>MDEKKLFLKALKKKFEGEDPDEKYTNFYCFGGWEQSARKKEFTEYAKKAAEKRGGIPFYNPDIGVPLGQRKLMAYRVSGTDAYVEGDDLHFVNNAAIQQMVDDIKRTVIVGMDTAHAVLEKRLGVEVTPETINEYMEAINHALPGGAVVQEHMVEVHPGLVEDCYAKIFTGDDNLADELDKRILIDINKEFPEEQAEQLKSYIGNRTYQVNRVPTIVVRTCDGGTVSRWSAMQIGMSFISAYKLCAGEAAIADFSYAAKHADVIEMGTIMPARRARGPNEPGGVAFGTFADIVQTSRVSDDPANVSLEVIAGAAALYDQVWLGSYMSGGVGFTQYATAAYTDDILDDFVYYGMEYVDDKYGICGTKPTMDVVRDISTEVTLYSLEQYEEYPTLLEDHFGGSQRAAVAAAAAGCSTAFATGNSNAGINGWYLSQILHKEAHSRLGFYGYDLQDQCGASNSLSIRSDEGLIHELRGPNYPNYAMNVGHQPEYAGIAQAPHAARGDAFCTNPLIKVAFADKDLAFDFTSPRKSIAAGALREFMPEGERDLIIPAGK[4x];>[4x]MPMYEDRIDLYGADGKLLEEDVPLEAISPLKNPTIANLVSDVKRSVAVNLAGIEGSLRKAALGGKSNFIPGREVELPIVENAEAIAEKVKKLVQTSEDDDTNIRLINNGQQILVQVPTTRMGVAADYTVSALVTGAAVVQAIIDEFDVDMFDANAVKTAVMGRYPQTVDFTGANLSTLLGPPVLLEGLGYGLRNIMANHVVAITRKNTLNASALSSILEQTAMFETGDAVGAFERMHLLGLAYQGLNANNLLFDLVKENGKGTVGTVIASLVERAVEDGVVKVAREMNSGYKVYEPADWALWNAYAATGLLAATIVNVGAARAAQGVASTVLYYNDILEYETGLPGVDFGRAMGTAVGFSFFSHSIYGGGGPGIFHGNHVVTRHSKGFALPCVAAAMCLDAGTQMFSVEKTSGLIGSVYSEIDYFREPIVNVAKGAAEVKDQL;>MSYKAQYTPGETQIAENRRKHMDPDYEFRKLREVSDEDLVKVLGHRNPGESYKSVHPPLDEMDFEEDIVRDMVEPIQGAKEGVRVRYIQFADSMYNAPAQPYDRARTYMWRYRGVDTGTLSGRQVIEMRELDLEGVSKELVETELFDPATTGIRGATVHGHSLRLDENGLMFDALQRYVFDEEKGHVVYVKDQVGRPLDEPVDMGQPLGE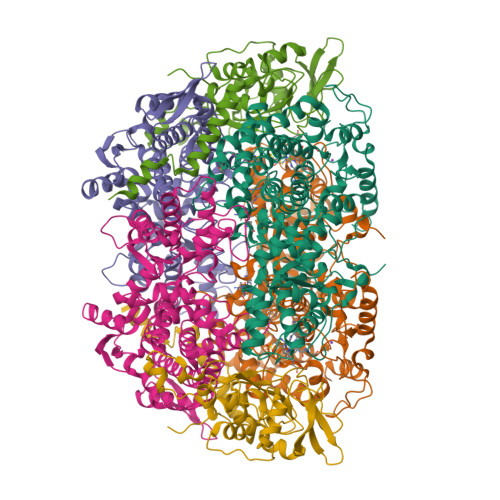DELKKITTIYRKDNIAMRDDKEAIEVVENIHTGRTLGGFGMDVFKDDLRKRLGDD[4x]MpPA14 (Marinomonas primoryensis PA14 domain) lectin is a domain of a 1.5-MDa adhesin responsible for a symbiotic bacterium-diatom interaction in Antarctica. Bioinformatic analyses indicated the presence of an ∼20-kDa domain near the C terminus of MpIBP that is a member of the PA14 family, which is a carbohydrate-binding lectin module widely distributed across several kingdoms of life. PA14 domains share a β-sandwich fold and the presence of two consecutive aspartate residues in a cis peptide linkage (DcisD). The DcisD motif coordinates a Ca2+ ion that is directly involved in binding polar vicinal hydroxyl groups of various carbohydrates.

Glucose and 2-deoxy-glucose bound the lectin with similar affinity, giving Kdapp values of 1.36 and 1.37 mM, respectively. d-Mannose and methyl-α-d-glucose bound MpPA14 with slightly weaker affinity (Kdapp = 1.7 mM and 2.1 mM, respectively), and the binding of d-allose, 3-O-methyl-d-glucose and d-galactose was significantly diminished to Kdapp values between 4.1 and 6.8 mM. Glucose, GlcNAc, and other glucopyranose-containing carbohydrates, including 2-deoxy-glucose, methyl-α-glucose, and two disaccharides (sucrose and trehalose), all bound to the Mp-PA14-Ca1 via their trans vicinal 3,4-diols (ionic bond length, 2.5 Å) in gauche configuration with a dihedral angle of ∼60°. This interaction is further enhanced with the diol being coordinated by the side chain carboxyl and hydroxyl oxygens of the DcisD motif, and main-chain and side chain protein ligands from L11 (Gln156, Gly157, and Asp159).

> AQDDSTPDSLFAGLVGEYYGTNSQLNNISDFRALVDSKEADATFEAANISYGRGSSDVAKGTHLQEFLGSDASTLSTDPGDNTDGGIYLQGYVYLEAGTYNFKVTADDGYEITINGNPVATVDNNQSVYTVTHASFTISESGYQAIDMIWWDQGGDYVFQPTLSADGGSTYFVLDSAILSSTGETPYTTAQ>MARPLEQAVAAIVCTFQEYAGRCGDKYKLCQAELKELLQKELATWTPTEFAECDYNKFMSVLDTNKDCEVDFVEYVRSLACLCLYCHEYFKDCPSEPPCSQ[2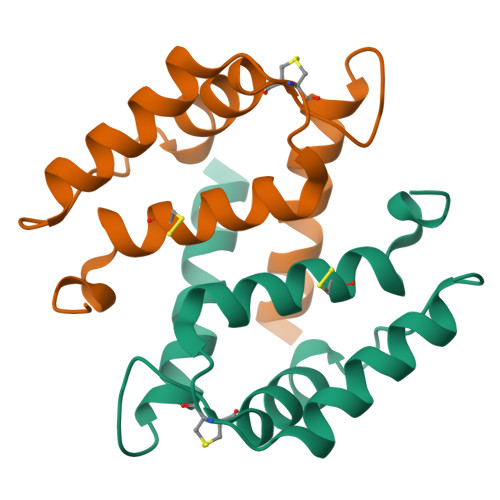x]>[2x]MSQSAPVNRPRLLTVKHIQDVSPHLRRICLTSPELADYPFTCGGAHIKIMLPQPGQAHAVLPTPTPQGPRWEDPSQRPIMRTFTIRAFRREALELDIDFALHGDGGPASRFANEVKPGDLLAISGPGGSDPMLQPASHYY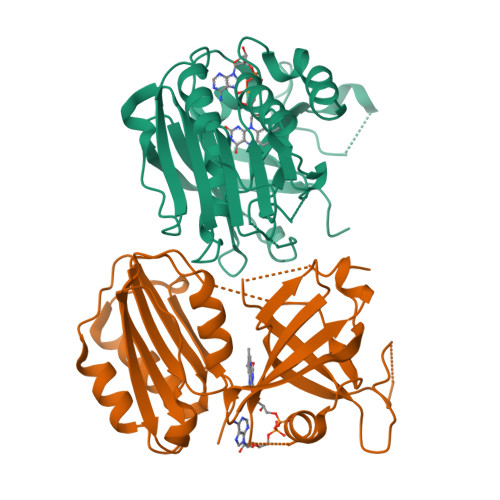MVGDLTALPAISAMAEVMPADARGHIALLVPYQEDVQDLSLPAGVTLRWFVGSPEETAPLVEYFTSLPLEEQQSYFWFGGEEGLVVPMRRHVRRTLEVDRTRVYAVPYWRHGKDEEAYHHARHDVMDS>[4x]GSMEKAAVNEDGLVIPLIDFSKFLEGDETLKLETAKAILHGFQTAGFIYLKNIPIQPDFREHVFNTSAKFFKLPKEKKLEVGWTTPEANRGYSAPGREKVTQLTDPAEIEKIRSAAPDIKESYEIGREDEPGHPNPWPAEQDDLVGFKSTMNNFFDQCKALHIEVMRAIAVGMGIDANYFDSFVDVGDNILRLLHYPAVKSEVFKINPGQVRAGEHTDYGSITLLFQDSRGGLQVKSPNGQFIDATPIENTVVVNAGDLLARWSNDTIKSTVHRVVEPPKQEDVHPPRYSIAYFCNPNHKSYIEAIPGTYAAESERKYEGINSGKYLVQRLAATYLEHHHHHH

Like the TET proteins, T7H is also a Fe2+ and α-KG dependent dioxygenase. Here we report the crystal structures of N. crassa T7H (NcT7H) in apo form, in α-KG-bound form and in complexes with α-KG and T, 5hmU or 5fU. Similar to other α-KG dependent dioxygenases, NcT7H adopts a variation of double-stranded β-helix (DSBH) fold as the core. The active site of NcT7H is located at the front end (opposite to the back end) of the DSBH core and partially covered by the α10 helix at the C-terminus.

The crystal structures of the full-length NcT7H in complex with α-KG (NcT7H-AKG), and in complexes with α-KG and T (NcT7H-T), with α-KG and 5hmU (NcT7H-5hmU), and with α-KG and 5fU (NcT7H-5fU) were solved by the MR method at 2.1 Å, 2.05 Å, 2.35 Å, and 2.15 Å resolution, respectively. In the substrate-bound NcT7H structures, T, 5hmU or 5fU binds to a pocket adjacent to the metal ion and α-KG, and has largely hydrophobic interactions and a few hydrophilic interactions with the surrounding residues. In the NcT7H-5hmU and NcT7H-5fU complexes, the uracil moiety of 5hmU or 5fU maintains almost identical interactions with the surrounding residues as that in the NcT7H-T complex. The C51 atom of 5hmU and 5fU is located about 3.7 Å and 3.9 Å away from the C1-carboxylate of α-KG, respectively. In addition, the 5-hydroxymethyl group of 5hmU or the 5-formyl group of 5fU forms a hydrogen bond with the C1-carboxylate of α-KG and a hydrogen bond with the side chain of Arg190. In the substrate-bound NcT7H structures, the side chain of Arg190 makes hydrogen-bonding interaction and/or van der Waals contacts with both the C1-carboxylate of α-KG and the C5 modification group of the substrate. In the substrate-bound NcT7H structures, the C1-carboxylate and C2-oxo groups of α-KG are located in opposite to His271 and Asp216 of the HXD/E…H motif, respectively, and Wat1 (which occupies presumably the oxygen in catalysis) is located below the plane formed by the C1-carboxylate of α-KG, Asp216 and His271 and in opposite to His214, indicating that the α-KG binding assumes the ‘off-line’ mode in NcT7H. NcT7H exhibits comparable Km and kcat values towards T and 5hmU but displays about 1.8-fold higher Km value and 2-fold higher kcat value towards 5fU, and the catalytic efficiency of NcT7H towards different substrates is in the order of 5fU ≥ T >5hmU, which are consistent with our binding affinity and activity assay results. The side chain of Tyr217 makes hydrophobic interactions with the substrates; mutation Y217F has insignificant effects on the activity towards T and 5hmU but a moderate effect on the activity towards 5fU, and mutation Y217A has moderate effects on the activity towards T and 5hmU but abolishes the activity towards 5fU. Additionally, these mutations abolish the activity for 5fU, leading to undetectable Km and kcat values.2-indol-1-ylethanoic acid 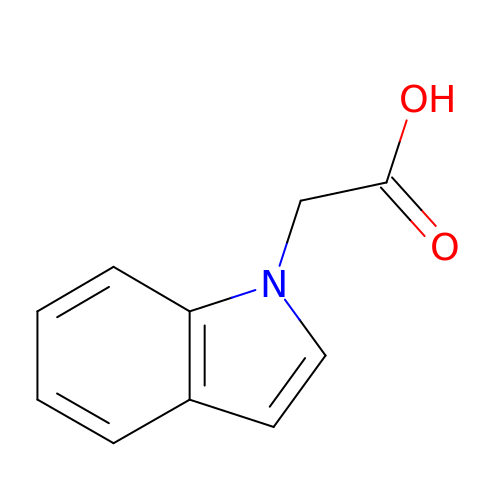| C10 H9 N O2 | WQJFIWXYPKYBTO-UHFFFAOYSA-N>[3x]GTKEVTSTNDDPLTPLNRFDKYYLRMFKKVPRLQQNGSNIINGVNMKNTVIVLYFFAKWCQACTMQSTEM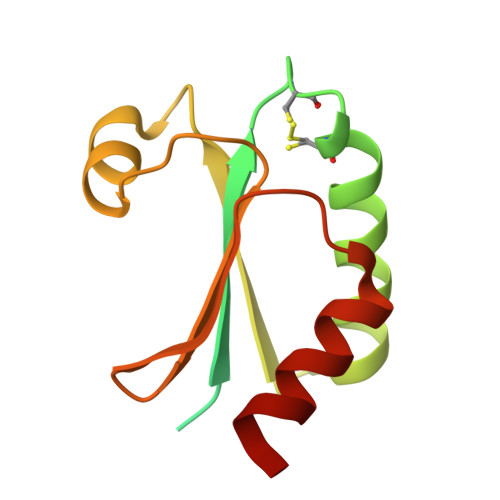DKLQKYYGKRIYLLKVDLDKNESLARKFSVKSLPTIILLKNKTMLARKDHFVSSNDLIALIKKHLVPR(5R)-5-[(5-methoxy-3-oxo-1,3-dihydro-2H-indazol-2-yl)methyl]-5-phenylimidazolidine-2,4-dione 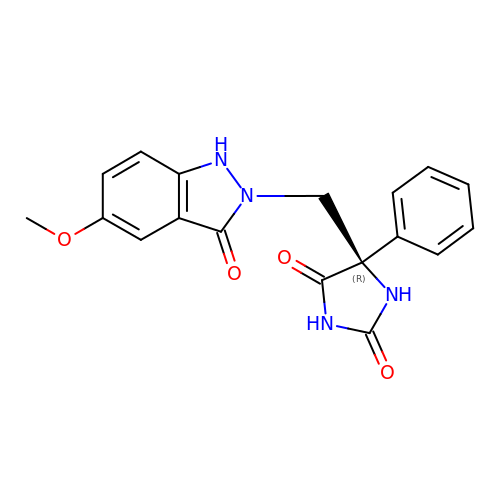| C18 H16 N4 O4 | OXEVTLWXFDHNQD-SFHVURJKSA-N> GSMRHILERPDPTDVFQNKANVCWAKALVPVLKTAGIDMTTEQWNTVDYFETDKAHSAEIVLNQLCVRFFGLDLDSGLFSAPTVPLSIRNNHWDNSPSPNMYGLNKEVVRQLSRRYPQLPRAVATGRVYDMNTGTLRNYDPRINLVPVNRRLPHALVLHHNEHPQSDFSSFVSKLKGRTVLVVGEKLSVPGKMVDWLSDRPEATFRARLDLGIPGDVPKYDIIFVNVRTPYKYHHYQQCEDHAIKLSMLTKKACLHLNPGGTCVSIGYGYADRASESIIGAIARQFKFSRVCKPKSSLEETEVLFVFIGYDRKARTHNPYKLSSTLTNIYTGSRLHEA

The Venezuelan equine encephalitis virus (VEEV) nonstructural protein 2 (nsP2) cysteine protease (EC 3.4.22.B79) is essential for viral replication. The nsP2 cysteine protease (nsP2pro, EC 3.4.22.B79) cleaves the polyprotein at three sites to produce four functional replication proteins. The cleavage is essential to replication and the alphaviral nsP2 cysteine protease has been validated as a drug target by deletion and mutation. VEEV contains a single-stranded positive-sense RNA ((+)ssRNA) genome and is a member of the alphavirus genus.

To examine the differences in inhibitor specificity, the CA074-inhibited VEEV nsP2 protease was crystallized. Here, we determined the X-ray crystal structure of the CA074-inhibited nsP2 protease and compared it with our E64d-inhibited structure. While the compounds appear similar, the regions occupied by the inhibitors differ. Notably, the two inhibitors occupy different locations in the protease. Notably, these two inhibitors occupy the subsites which bind the most highly conserved residues of alphaviral protease substrates. The histidine of the catalytic dyad rotates towards the inhibitor when the active site becomes occupied. CA074 makes 8 h bonds to the enzyme. Rates of inactivation by CA074 in the presence of 6 mM CaCl2, MnCl2, or MgCl2 were measured with varying concentrations of inhibitor, Mg2+ and Mn2+ slightly enhanced inhibitor binding (3 to 6-fold). CA074 inhibited not only the VEEV nsP2 protease but also that of CHIKV and WEEV.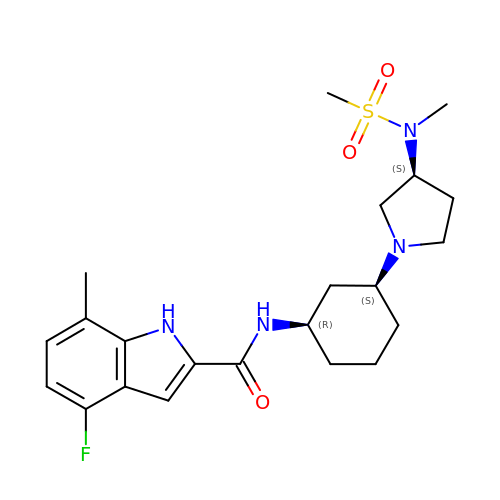4-fluoro-N-[(1R,3S)-3-{(3S)-3-[(methanesulfonyl)(methyl)amino]pyrrolidin-1-yl}cyclohexyl]-7-methyl-1H-indole-2-carboxamide | C22 H31 F N4 O3 S | ZLVKIBLQXFILMA-IKGGRYGDSA-N> MERLWKDIKRDWLLYAMLLPTIIWFLIFLYKPMIGLQMAFKQYSAWKGIAGSPWIGFDHFVTLFQSEQFIRAIKNTLTLSGLSLLFGFPMPILLALMINEVYSKGYRKAVQTIVYLPHFISIV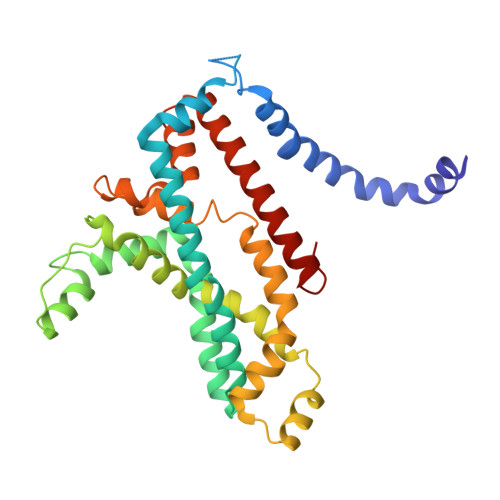IVAGLVVTFLSPSTGVVNNMLSWIGLDRVYFLTQPEWFRPIYISSNIWKEAGFDSIVYLAAIMSINPALYESAQVDGATRWQMITRITLPCIVPTIAVLLVIRLGHILEVGFEYIILLYQPTTYETADVISTYIYRLGLQGARYDIATAAGIFNAVVALVIVLFANHMSRRITKTGVF>[2x]GMETTDTKREEQEIEEKKAQEESKIEDVDKILNDILSISSECIQPDELRVKLLLKRKLICYDGFEPSGRMHIAQGLLKSIIVNKLTSNG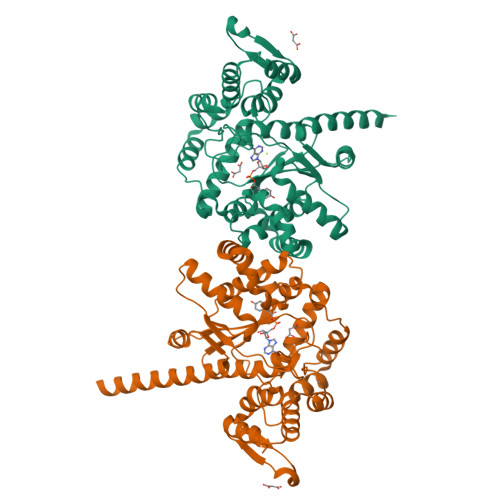CTFIFWIADWFAHLNNKMSGDLKKIKKVGSYFIEVWKSCGMNMENVQFLWASEEINKKPNEYWSLVLDISRSFNINRMKRCLKIMGRSEGEENYCSQILYPCMQCADIFFLNVDICQLGIDQRKVNMLAREYCDIKKIKKKPVILSHGMLPGLLEGQEKMSKSDENSAIFMDDSESDVNRKIKKAYCPPNVIENNPIYAYAKSIIFPSYNEFNLVRKEKNGGDKTYYTLQELEHDYVNGFIHPLDLKDNVAMYINKLLQPVRDHFQNNIEAKNLLNEIKKYKVTK>[3x]GSHM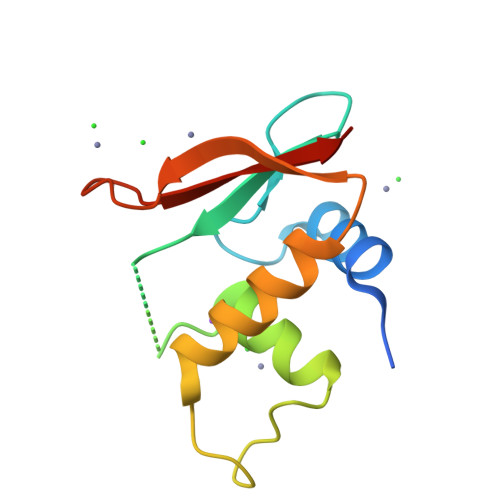GTPKPRILPWLVSQLDLGQLEGVAWVNKSRTRFRIPWKHGLRQDAQQEDFGIFQAWAEATGAYVPGRDKPDLPTWKRNFRSAMNRKEGLRLAEDRSKDPHDPHKIYEFVNSG2-amino-2-deoxy-beta-D-galactopyranose 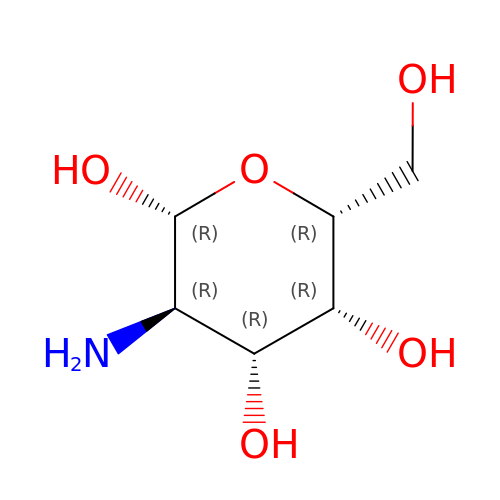| C6 H13 N O5 | MSWZFWKMSRAUBD-VFUOTHLCSA-N>MGKVPHIRIENGAAIEEIYTFGRILGKGSFGIVIEATDKETETKWAIKKVNKEKAGSSAVKLLER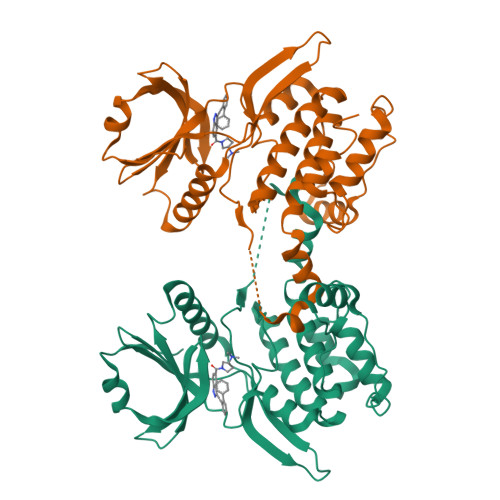EVNILKSVKHEHIIHLEQVFETPKKMYLVMELCEDGELKEILDRKGHFSENETRWIIQSLASAIAYLHNNDIVHRDLKLENIMVKSSLIDDNNEINLNIKVTDFGLAVKKQSRSEAMLQATCGTPIYMAPEVISAHDYSQQCDIWSIGVVMYMLLRGEPPFLASSEEKLFELIRKGELHFENAVWNSISDCAKSVLKQLMKVDPAHRITAKELLDNQWLTG[2x]>[2x]HHHHHHFNLPPGNYKKPKLLYC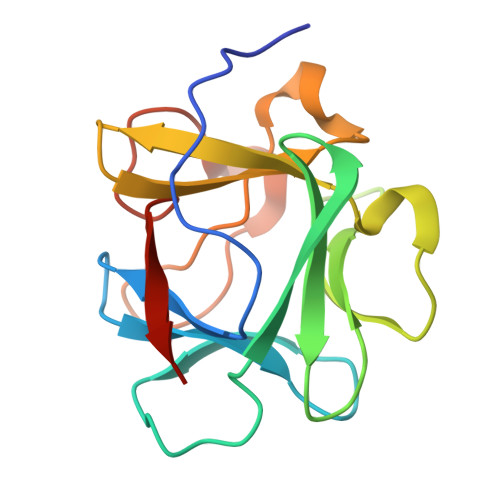SNGGHFLRILPDGTVDGTRDRSDQHIQLQLSAESVGEVYIKSTETGQYLAMDTDGLLYGSQTPNEECLFLERLEENHYNTYISKKHAEKNWFVGLNKNGSCKRGPRTHYGQKAILFLPLPVSSD> MDVSILGTGLMGTALAQALIRSGTKVTVWNRTADRALPLAAAGATVAESPQSAIAASPLIVISLLNYEIAKDVVTEADSIAGKIIVNTATGTPEEANQFAEWIAGRGARYLDGAIAAYPEDIGTESSGINYSGDEDVWEDVQSLLTPIAAQSRYVGARPGAANVIDAAMAGAFFNVALGAFHEAAAYVRSEDVAIAEMRHSLHLWTDKLLELLHEALKAFESGEYETDQATLNVYAAAVEAWQQSMQRAGQRAALMTANLDNLQRACAAGHGDKGIFAQIETLSANPQSAI

Here, we describe the discovery and synthetic potential of an IRED from Rhodococcus erythropolis (RytRedAm) that catalyzes reductive amination between a series of medium to large carbonyl and amine compounds with conversions of up to >99% and 99% enantiomeric excess at neutral pH. IREDs are homodimeric enzymes that contain a Rossmann-fold and prefer NADPH over NADH. RytRedAm catalyzes the formation of a substituted γ-lactam and N-methyl-1-phenylethanamine with stereochemistry opposite to that of fungal RedAms, giving the (S)-enantiomer. This enzyme remarkably uses both NADPH and NADH cofactors with KM values of 15 and 247 μM and turnover numbers kcat of 3.6 and 9.0 s–1, respectively, for the reductive amination of hexanal with allylamine. Considering the key amino acids involved in the active site, we propose the following mechanism based on previous observations with AspRedAm.22 Y235 would be involved as a proton donor, while D166 and T90 coordinate the protonated amine donor.

In an effort to shed light on the determinants of cofactor binding by RytRedAm, its structure was determined by X-ray crystallography in two forms. Each structure was obtained in space group P3221 with one molecule in the asymmetric unit; therefore, the IRED dimer was constructed using the symmetry neighbor. While cocrystallization with NAD+ or NADP+ failed to give a structure with a fully intact cofactor, crystals obtained with the latter gave an ADP-2′-ribose phosphate (ADP-2RP) complex (density for the nicotinamide ring and ribose sugar of NADP+ being absent) that revealed the residues involved in cofactor binding. At first glance, the cofactor binding motif in the RytRedAm sequence is similar to other IREDs/RedAms that have strong NADPH preference. RytRedAm already has an R in position 35 equiv to 37; in the structure of RytRedAm in complex with ADP-2RP, the side chain had incomplete density for the terminal guanidinium group, but the map at a level of 0.6 σ indicates that the side chain is pointing away from the phosphate binding site. The crystal structure obtained provides insights into the flexibility to also accept NADH, with residues R35 and I69 diverging from that of other IREDs/RedAms in the otherwise conserved Rossmann fold. A consideration of the variant data suggests that the preference for either cofactor is a complicated phenomenon with synergistic input from a number of residues, but the observations for RytRedAm may provide useful indicators for the mutations of other IREDs to alter cofactor specificity.>MGSDKIHHHHHHENLYFQGMINEQRLLNTFLELVQIDSETGNESTIQPILKEKFIALGLDVKEDEAAKHPKLGANNLVCTMNSTIEEGEVPKLYLTSHMDTVVPAINVKPIVKDDGYIYSDGTTILGADDKAGLAAMLEVLQVIKEQQIPHGQIQFVITVGEESGLIGAKELNSELLDADFGYAIDASADVGTTVVGAPTQMLISAKIIGKTAHASTPKEGVSAINIAAKAISRMKLGQVDEITTANIGKFHGGSATNIVADEVILEAEARSHDPERIKTQVKHMTDVFETTASELGGKAEVTVEQSYPGFKINDNEAVVKIAQESARNLGLSANTIISGGGSDGSIINTFGIPSVILGVGYEKIHTTNERMPIKSLNLLASQV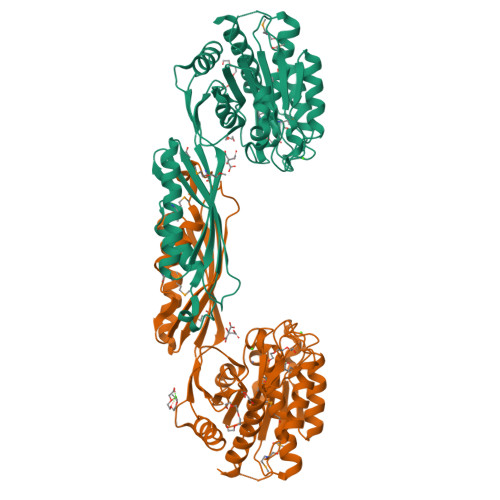LEIIKIVARQSK[2x]>MKFGKKLGFLALLMSIVLILGACGKTGLGNSSENSTKNVTKKSAKDLKLGVSISTTNNPYFVAMKDGIDKYASNKKISIKVADAQDDAARQADDVQNFISQNVDAILINPVDSKAIVTAIKSANNANIPVILMDRGSEGGKVLTTVASDNVAAGKMAADYAVKKLGKKAKAFELSGVPGASATVDRGKGFHSVAKSKLDMLSSQSANFDRAKALNTTQNMIQGHKDVQIIFAQNDEMALGAAQAVKSAGLQNVLIVGIDGQPDAHDAIKKGDISATIAQQPAKMGEIAIQAAIDYYKGKKVEKETI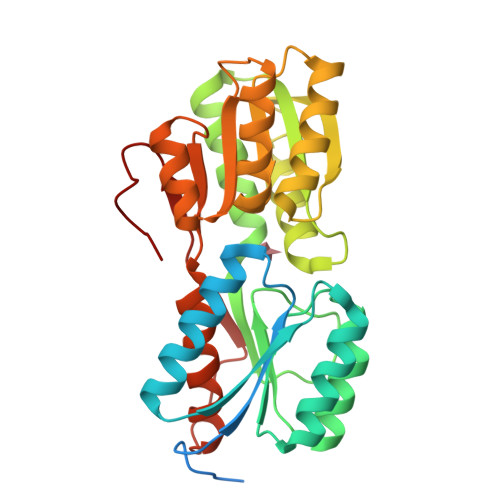SPIYLVTKDNVEKYNW[4x]~{N}-[(2~{S})-3-(1~{H}-indol-3-yl)-1-(methylamino)-1-oxidanylidene-propan-2-yl]-8-[2-methoxy-5-(trifluoromethyloxy)phenyl]-1,6-naphthyridine-2-carboxamide 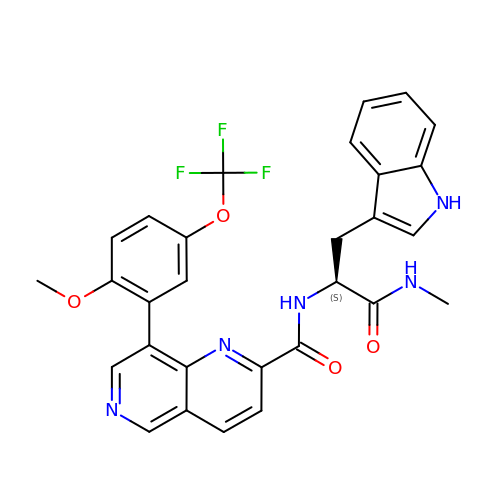| C29 H24 F3 N5 O4 | HXNJLYFKGOKJJR-DEOSSOPVSA-N> DLKCVTNNLQVWQCSWKAPSGTGRGTDYEVCIEQRSRSCYQLEKTSIKIPALSHGDYEITINSLHDFGSSTSKFTLNEQNVSLIPDTPEILQLSADFSTSTLYLKWNDRGSVFPHRSNVIWEIKVLRKESMELVKLVTHQTTLNGKDTLHHWSWASDMPLECAIHFVEIRCYIDNL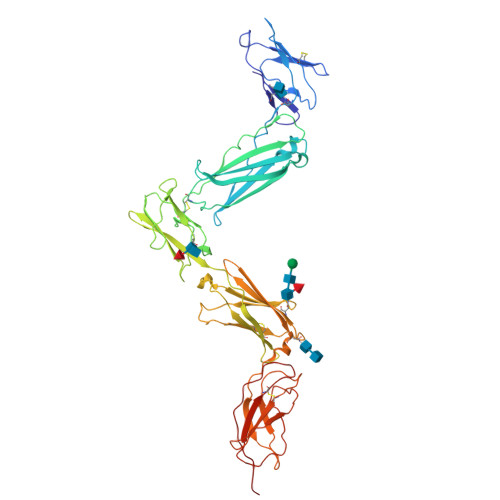HFSGLEEWSDWSPVKQISWIPDSQTKVFPQDKVILVGSDITFCCVSQEKVLSALIGHTNCPLIHLDGENVAIKIRNISVSASSGTNVVFTTEDNIFGTVIFAGYPPDTPQQLNCETHDLKEIICSWNPGRVTALVGPRATSYTLVESFSGKYVRLKRAEAPTNESYQLLFQMLPNQEIYNFTLNAHNPLGRSQSTILVNITEKVYPHTPTSFKVKDINSTAVKLSWHLPGNFAKINFLCEIEIKKSNSVQEQRNVTIQGVENSSYLVALDKLNPYTLYTFRIRCSTETFWKWSKWSNKKQHLTTEAS>MGSTEYKPTVRLATRDDVPRAVRTLAAAFADYPATRHTVDPDRHIERVTELQELFLTRVGLDIGKVWVADDGAAVAVWTTPESVEAGAVFAEIGPRMAELSGSRLAAQQQMEGLLAPHRPKEPAWFLATVGVSPDHQGKGLGSAVVL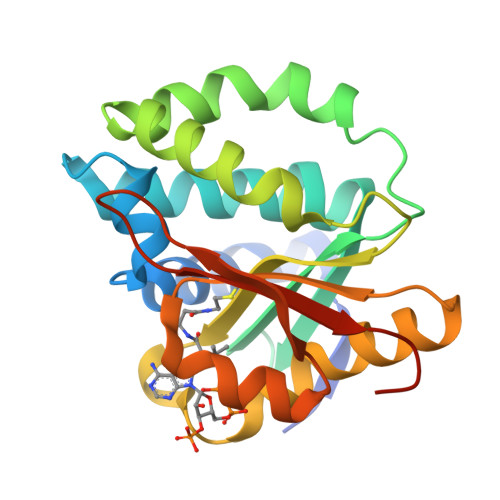PGVEAAERAGVPAFLETSAPRNLPFYERLGFTVTADVEVPEGPRTWCMTRKPGASHHHHHH[6x]> MASSRRESINPWILTGFADAEGSFLLRIRKNNKSSVGYSTELGFQITLHNKDKSILENIQSTWGVGVIANSGDNAVSLKVTRFEDLKVIIDHFEKYPLITQKYADYMLFKQAFNVMENKEHLTIEGIKELVR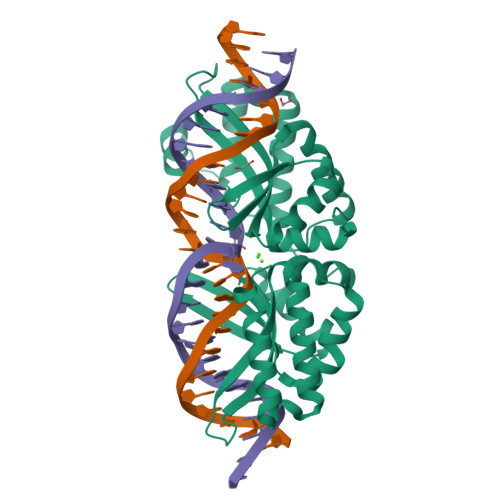IKAKLNWGLTDELKKAFPEIISKERSLINKNIPNFKWLAGFTSGDGCFFVNLIKSKSKLGVQVQLVFSITQHIRDKNLMNSLITYLGCGYIKKKNKSEFSWLDFVVTKFSDIRDKIIPFFQEYTLIGTKLKDFEDWCKVAKLIEEKKHLTEEGLDEIKKIKLNMNKGRVF2-[2,5-bis(oxidanylidene)imidazolidin-1-yl]-~{N}-[4-bromanyl-3-[(3~{S})-3-methylpiperidin-1-yl]sulfonyl-phenyl]ethanamide 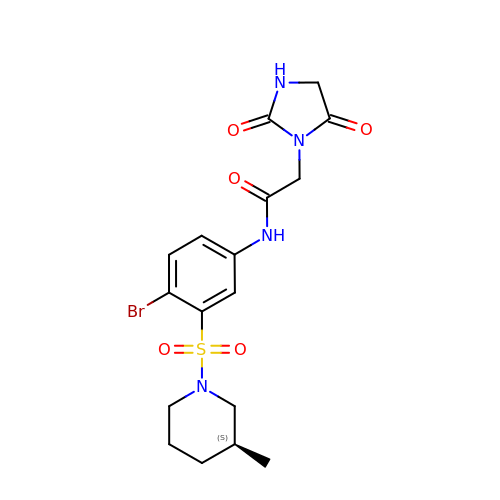| C17 H21 Br N4 O5 S | ANTNWJRSPNQTEF-NSHDSACASA-N>[32x]MGRMLGRKERTLTYLGPDTEVLGDMRA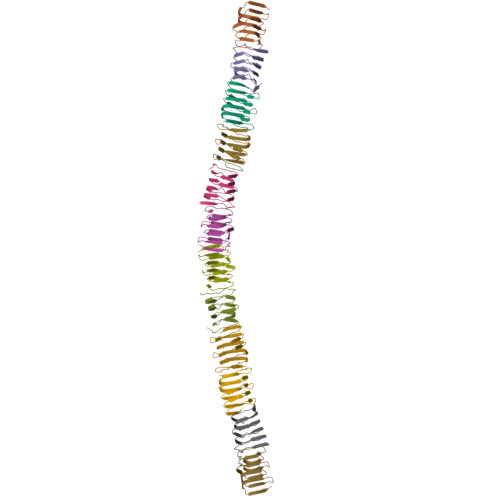KGQVRIDGLVRGSVLVEGELEVGPTGRVEGERVEARSVLIHGEVKAELTAEKVVLSKTARFTGQLKAQALEVEAGAVFVGQSVAGEHKALEAPKEA>GSSHHHHHHSQDPAPTLLTTQFSNPAEVTDFVVYKGNGVKGLSETGIKALPEQYIQPLEERLINKFVNETDEAIPVIDMSNPDEDRVAEAVCDAAEKWGFFQVINHGVPLEVLDDVKAATHKFFNLPVEEKRKFTKENSLSTTVRFGTSFSPLAEQALEWKDYLSLFFVSEAEAEQFWPDICRNETLEYINKSKKMVRRLLEYLGKNLNVKELDETKESLFMGSIRVNLNYYPICPNPDLTVGVGRHSDVSSLTILLQDQIGGLHVRSLASGNWVHVPPVAGSFVINIGDAMQIMSNGLYKSVEHRVLANGYNNRISVPIFVNPKPESVIGPLPEVIANGEEPIYRDVLYSDYVKYFFRKAHDGKKTVDYA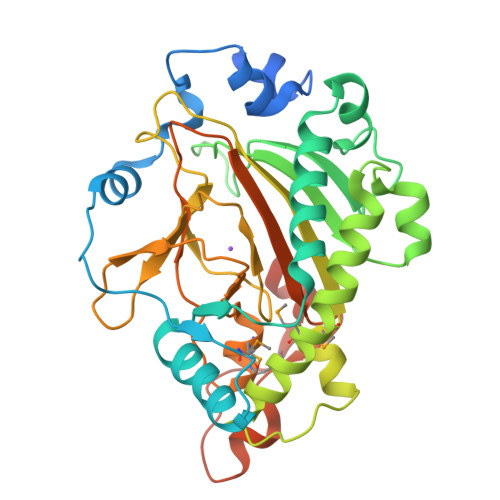KI[2x]> GSLYNDGNRDQRNFGRNQRNNNSNRYRNSRFNSRPRTRSREDDDEVHFDKTTFSKLIHVPKEDNSKEVTLDSLLEEGVLDKEIHKAITRMEFPGLTPVQQKTIKPILSSEDHDVIARAKTGTGKTFAFLIPIFQHLINTKFDSQYMVKAVIVAPTRDLALQIEAEVKKIHDMNYGLKKY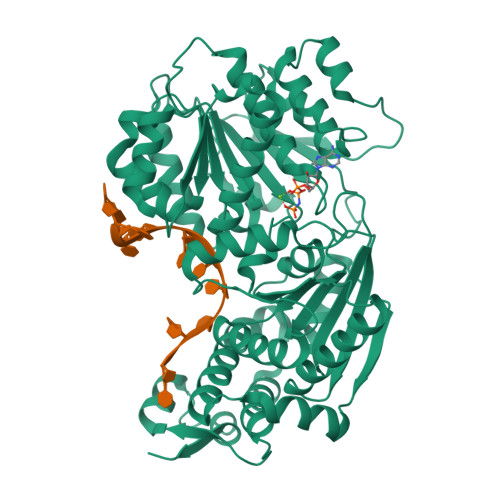ACVSLVGGTDFRAAMNKMNKLRPNIVIATPGRLIDVLEKYSNKFFRFVDYKVLDEADRLLEIGFRDDLETISGILNEKNSKSADNIKTLLFSATLDDKVQKLANNIMNKKECLFLDTVDKNEPEAHERIDQSVVISEKFANSIFAAVEHIKKQIKERDSNYKAIIFAPTVKFTSFLCSILKNEFKKDLPILEFHGKITQNKRTSLVKRFKKDESGILVCTDVGARGMDFPNVHEVLQIGVPSELANYIHRIGRTARSGKEGSSVLFICKDELPFVRELEDAKNIVIAKQEKYEPSEEIKSEVLEAVTEEPEDISDIVISLISSYRSCIKEYRFSERRILPEIASTYGVLLNDPQLKIPVSRRFLDKLGLSRSPIGKAMFEIRDY(2R)-2-phenyl-2-(phenylamino)-N-(1H-tetrazol-5-yl)acetamide | C15 H14 N6 O | 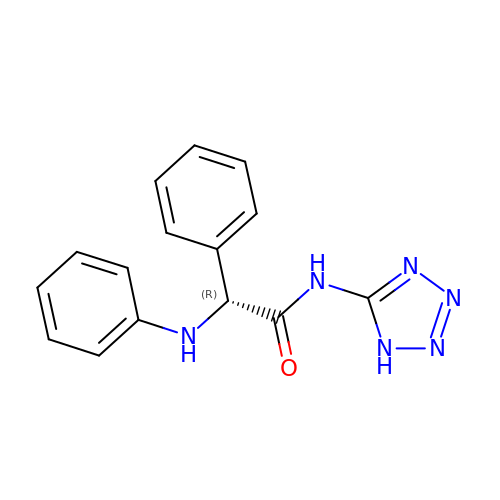PLRZYAQVTMJESZ-CYBMUJFWSA-N>MVLKLYAVSDGPPSLSVRQALVALEVPFELINVDFGAGEHMTSDYALMNPQKEIPVLDDEGFYLSESNAILQYICDKYRPGSPLYPQDPKSRAIVNHRLCFNLSSYYANISAYTMAPIFFDYERTPLGLKKVHISLDVLET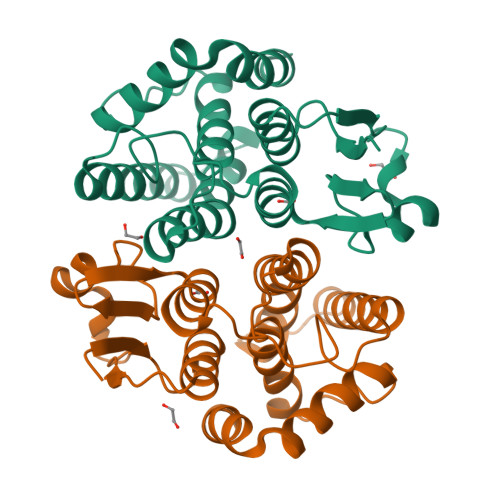YLTRTNTSYAAANHLTIADFPLINSTMTLEAIDFDFSKYTKIHKWYNDFKVKYPDLWKISESAMKEIQHFAANPPDLTHLNHPIHPIRKIKN[2x]> MTENILRKSDEEIQKEITARVKALESMLIEQGILTTSMIDRMAEIYENEVGPHLGAKVVVKAWTDPEFKKRLLADGTEACKELGIGGLQGEDMMWVENTDEVHHVVVCTLCDCYPWPVLGLPPNWFKEPQYRSRVVREPRQLLKEEFGFEVPPSKEIKVWDSSSEMRFVVLPQRPAGTDGWSEEELATLVTRESMIGVEPAKAV;> MNGVYDVGGTDGLGPINRPADEPVFRAEWEKVAFAMFPATFRAGFMG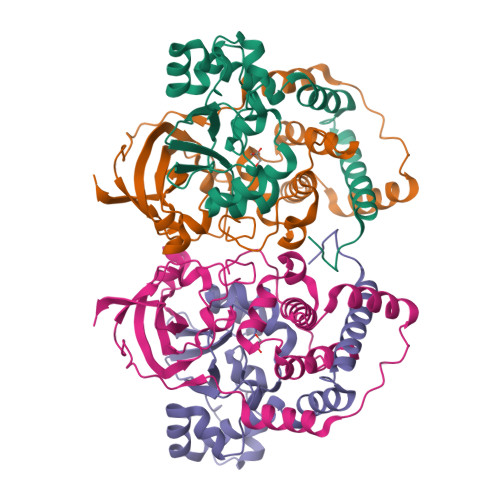LDEFRFGIEQMNPAEYLESPYYWHWIRTYIHHGVRTGKIDLEELERRTQYYRENPDAPLPEHEQKPELIEFVNQAVYGGLPASREVDRPPKFKEGDVVRFSTASPKGHARRARYVRGKTGTVVKHHGAYIYPDTAGNGLGECPEHLYTVRFTAQELWGPEGDPNSSVYYDCWEPYIELVDT> MGSSHHHHHHSSGLVPRGSHMSSSRSSSMDKTGWITHCFGRFLIDLPPDAVINAGYYLWGDRIEYLDDKPTELAARVDRLEQEWRTQRHKSKGNMFLRKIDFGNESVGLLSWSSEVASKTYLLDTYVTSKPTWHVYRWKGKVSVDREQHAVEISRALARNLRSRAPKEIPSEPGFCIDHAYIAGDSFQVERFGVGVTFPEHPGARFEFRSSTGAELNSLLERVDGFVQNMLSTFAGMETLRKGKHPVG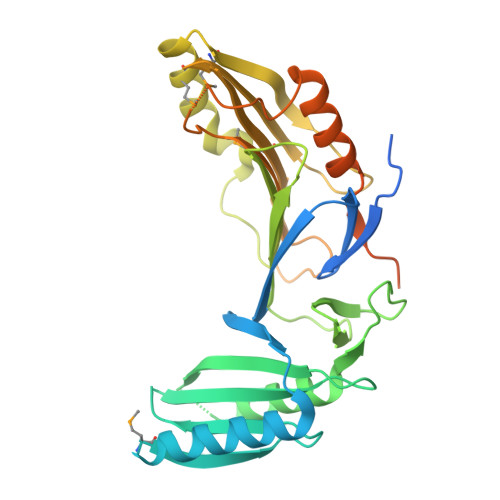SLPGEEYLVAGSDKGQRGYTFMWEVQGKEESLTEPNLTAGLAVLERSNENGKPPPPAFKSDKEALELWDTIVDSIRVRPTSSSPRGGNAGPSPAPKPATPGGQTLGDHYVYEEFLSSLKPKDSWLDDL HAL is a tetrameric enzyme that catalyzes the first step in histidine catabolism and thus is important for central metabolism; consequently, it exists in a wide variety of organisms from across the tree of life. We decided to use the enzyme histidine ammonia lyase (HAL), an enzyme from a family with broad synthetic and therapeutic applications, as a test case. Specifically, we demonstrate that the HAL enzyme originating from the archaeon Thermoplasma acidophilum is tolerant to both heat and acid stresses. Thermoplasma acidophilum histidine ammonia lyase was identified as an enzyme with a promising catalytic profile following acid treatment.

The crystal structure of TaHAL was solved, and we found that, similar to other members of the ammonia-lyase family, TaHAL crystallized as a homotetramer. Moreover, it exhibited electron density consistent with the MIO moiety known to provide catalytic activity in this enzyme class. Notably, there is a clear enrichment of negatively charged residues on the surface of the protein. It has been observed that an enrichment of negative charges on the surface of a protein can contribute to solubility and acid stability, and perhaps the observed enrichment of negative surface charges contributed to TaHAL’s resistance to acid and heat stresses. Measuring the temperature-dependent conversion of histidine to trans-urocanic acid by TaHAL in buffer A showed an increase in enzymatic activity with a maximal kcat at 60 °C. Upon heating the cuvette to 90 °C, only small changes in the absorbance at 222 nm and the spectrum as a whole were observed, indicating that the TaHAL protein retained much of its secondary structure even at high temperatures. The pH profile of TaHAL activity showed an optimum pH between pH 8 and 10. We found that TaHAL activity was well maintained with exposure to pH 4, but the activity decreased when TaHAL was incubated at pH 3 and below. Exposure to pH 2.8 allowed for the recovery of ~20% activity following neutralization, but 97% of the TaHAL activity was lost following 2 hours at pH 2.5. Upon titration with phosphoric acid, the protein appeared to maintain nearnative secondary structure until a pH of ~3, consistent with the observed partially irreversible loss of activity seen at pH levels below 4.

> SMIEIDGRSLRVEDVYAVAVEYDRVSISDDTLKAVEEKHEAFLKLINSGKTVYGVNTGFGSLLNVHIERDQEIELQKNLIRSHSSGVGDYLENRYVRAIMAVRLNSLAAGYSAVSADLLNMMVEMLNRDVIPAVPKYGSVGASGDLAPLAHIGLAMMGEGKAFFEGRLMDSARALEKAGLKPYQFKEKEGVALINGTSFMSGILSIAVMDAHDILENAIRSALLSFEALGGTSKAFTPWILGARPHLGQVAIGNRFREYLTGSDIVKRADSVKVQDAYTLRCIPQVYGSVADVIDYVENVLSVEINSATDNPLFNGEEVVSGGNFHGEPVALAADFLAIALTDLGNMVERRIARLVDTNLSGLPPFLTPDSGLNSGYMIPQYTAAALCNRNKVLAYPSSADTIPTSANQEDHVSMGATGSLKLLEIIDNVRYIIAIEYLLGSQALEFTDKGMSPSTRKIYEKIREKVEKLDHDRPPSFDIETIRKMMDKKEFISALP> HHHHHHMNKVLLLSIQNPLYPITVDVL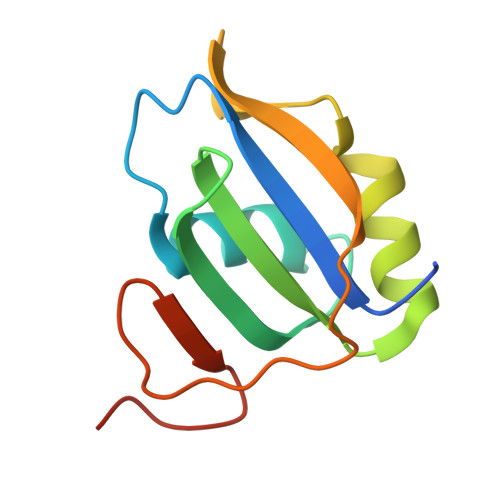YTVCNPVGKVQRIVIFKRNGIQAMVEFESVLCAQKAKAALNGADIYAGCCTLKIEYARPTRLNVIRNDNDSWDYTKPYLGRRD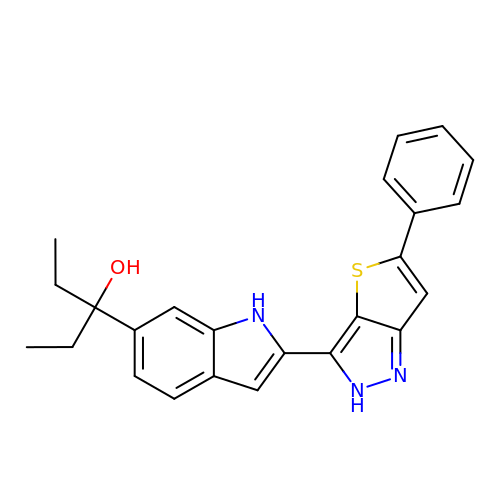3-[2-(5-phenyl-2H-thieno[3,2-c]pyrazol-3-yl)-1H-indol-6-yl]pentan-3-ol | C24 H23 N3 O S | YBKODNZGBUDZRA-UHFFFAOYSA-N>GSMSSERVLSYAPAFKSFLDTSFFQELSRLKLDVLKLDSTSQPLTVNLDLHNIPKSADQVPLFLTNRSFEKHNNKRTNEVPLQGSIFNFNVLDEFKNLDKQLFLHQRALECWEDGIKDINKCVSFVIISFADLKKYRFYYWLGVPCFQRPSSTVLHVRPEPSLKGLFSKCQKWFDVNYSKWVCILDADDEIVNYDKSIIRKTKVLAIRDTSTMENVPSALTKNFLSVLQYDVPDLIDFKLLIIRQNEGSFALNATFASIDPQSSSSNPDMKVSGWERNVQGKLAPRVVDLSSLLDPLKIADQSVDLNLKLMKWRILPDLNLDIIKNTKVLLLGAGTLGCYVSRALIAWGVRKITFVDNGTVSYSNPVRQALYNFEDAGKPKAELAAASLKRIFPLMDATGVKLSIPMIGHKLVNEEAQHKDFDRLRALIKEHDIIFLLVDSRESRWLPSLLSNIENKTVINAALGFDSYLVMRHGNRDEQSSKQLGCYFCHDVVAPTDSLTDRTLDQMCTVTRPGVAMMASSLAVELMTSLLQTKYSGSETTVLGDIPHQIRGFLHNFSILKLETPA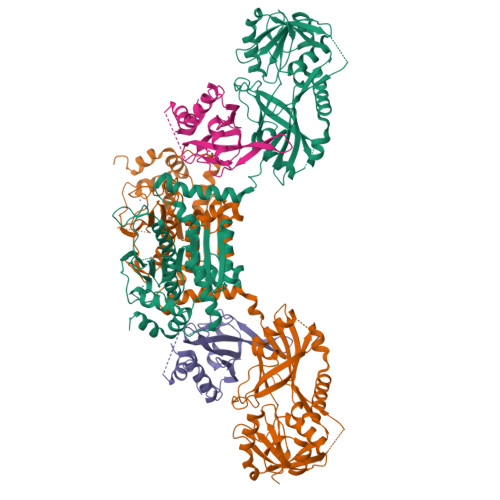YEHCPACSPKVIEAFTDLGWEFVKKALEHPLYLEEISGLSVIKQEVER[2x];>GSGGSGMIPYQEWHSQLQSLYDSQIFHNWALSQDVHLNDEKDGLLLRLIPTRQLQKNTERIENKLLNHIELYLTYSKVYNEPLLLLRIWEEKSIDGIPMTKLMLPTDIESLLDVQGKFQLGLDTIINLEGSVWYSFHPCDTSSIVGDQAEFMSTYLRRWVSIFIFSWLGYEDS[2x]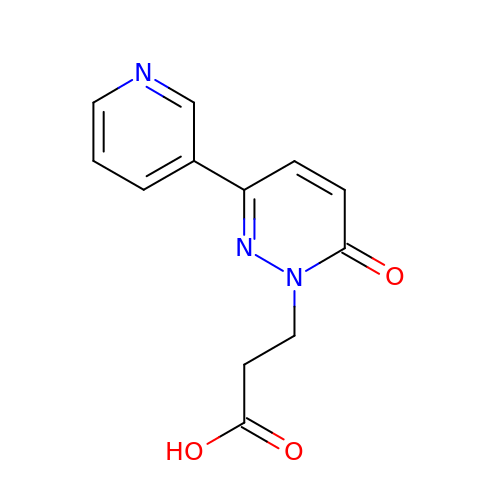3-(6-oxidanylidene-3-pyridin-3-yl-pyridazin-1-yl)propanoic acid | C12 H11 N3 O3 | FPHNPEYKDLCEEE-UHFFFAOYSA-N URIDINE-5'-DIPHOSPHATE-MANNOSE 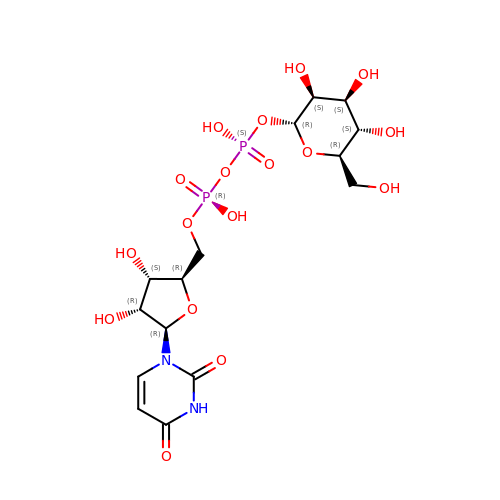| C15 H24 N2 O17 P2 | HSCJRCZFDFQWRP-NYYOCOOHSA-N> LLGDFFRKSKEKIGKEFKRIVQRIKDFLRNLVPRTE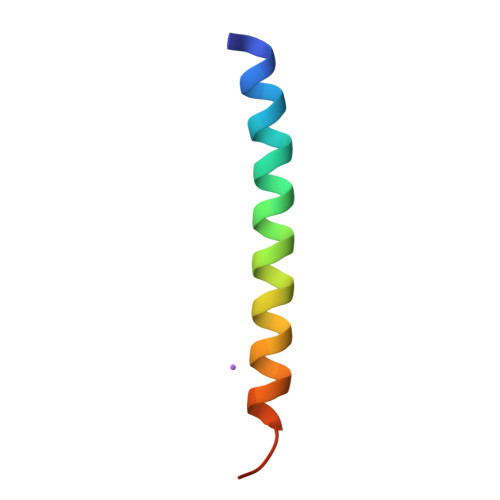S>[2x]MANVAKKVSWSGRDPRDDEDERAGETTPLLNGTGPGSAGGARQFTPSSFLRPGQLSNVDLNEDIRELETELPRPYPNEIPHNEKLLSLKYESLDYDNSENQLFLEEERRINHAAFRTVEIKRWVICAMIGILTGLVACFIDIVVENLAGLKYRVVKDNIDKFTEKGGLSFSLLLWATLNASVVMVGSVIVAFIEPVAAGSGIPQIKCYLNGVKIPHVVRLKTLVIKVCGVILSVVGGLAVGKEGPMIHSGAVIAAGISQGRSTSLKRDFKIFEYFRRDTEKRDFVSAGAAAGVSAAFGAPVGGVLFSLEEGASFWNQFLTWRIFFASMISTFTLNSVLSVYHGNAWDLSSPGLINFGRFDSEKMGYTIQEIPIFIFMGVVGGILGALFNALNYWLTMFRIRYIHRPCLQVIEAMLVAAVTAAVGFVMIYCSRDCQPIQGS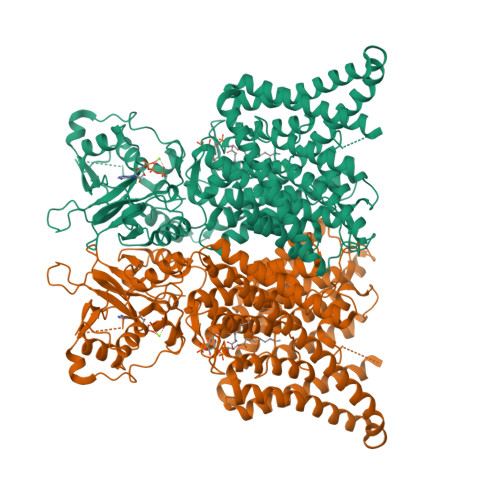SVAYPLQLFCADGEYNSMATAFFNTPEKSVVNLFHDPPGSYNPMTLGMFTLMYFFLACWTYGLTVSAGVFIPSLLIGAAWGRLFGISLSYLSKGSIWADPGKYALMGAAAQLGGIVRMTLSLTVIMMEATGNVTYGFPIMLVLMTAKIVGDYFVEGLYDMHIQLQSVPFLHWEAPVTSHSLTAREVMSTPVTCLRRIERVGTVVDILSDTSSNHNGFPVVESNPNTTQVAGLRGLILRSQLIVLLKHKVFVERANLNLVQRRLKLKDFRDAYPRFPPIQSIHVSQDERECMIDLSEFMNPSPYTVPREASLPRVFKLFRALGLRHLVVVNNHNEVVGMVTRKDLARYRLGKEGLEELSLAQT> MIQVTSEQWLYWLHLYFWPLLRVLALISTAPILSERAIPKRVKLGLGIMITLVIAPSLPANDTPLFSIAALWLAMQQILIGIALGFTMQFAFAAVRTAGEFIGLQMGLSFATFVDPGSHLNMPVLARIMDMLAMLLFLTFNGHLWLISLLVDTFHTLPIGSNPVNSNAFMALARAGGLIFLNGLMLALPVITLLLTLNLALGLLNRMAPQLSIFVIGFPLTLTVGIMLMAALMPLIAPFCEHLFSEIFNLLADIVSEMPINNN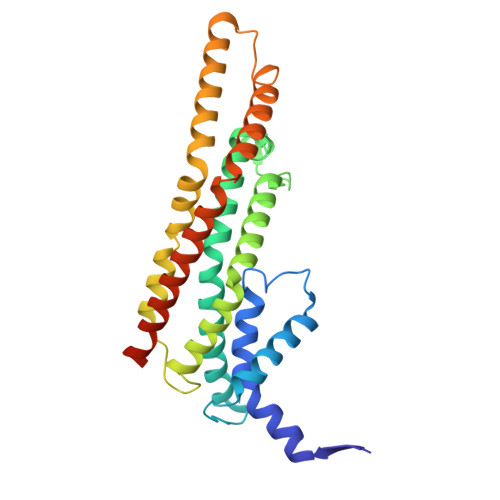PHHHHHHHHHH nonane | C9 H20 | 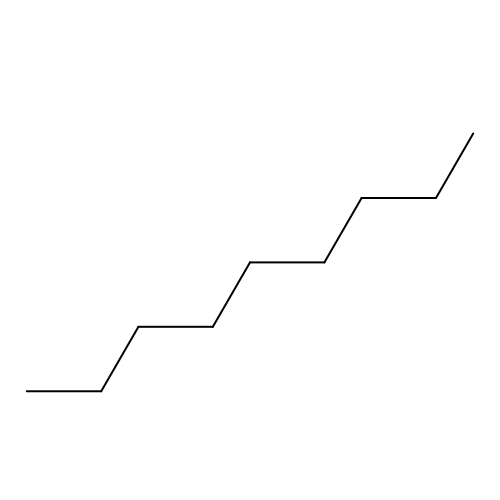BKIMMITUMNQMOS-UHFFFAOYSA-N> MHHHHHHHHTFTRYSRLRVIAEIRHGDIFHSANIVSSIEFDRDDELFATAGVSRCIKVFDFSSVVNEPADMQCPIVEMSTRSKLSCLSWNKHEKNH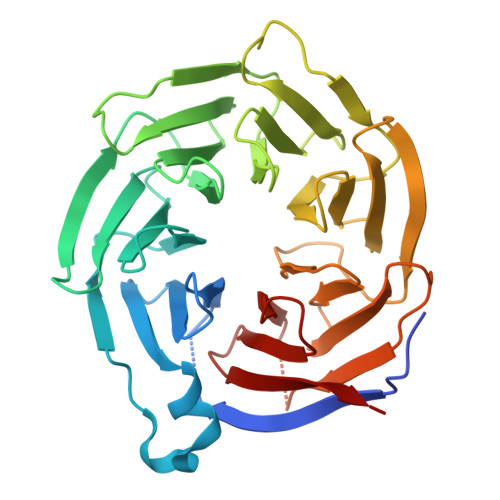IASSDYEGIVTVWDVTTRQSLMEYEEHEKRAWSVDFSRTEPSMLVSGSDDCKVKVWCTRQEASVINIDMKANICCVKYNPGSSNYIAVGSADHHIHYYDLRNISQPLHVFSGHKKAVSYVKFLSNNELASASTDSTLRLWDVKDNLPVRTFRGHTNEKNFVGLTVNSEYLACGSETNEVYVYHKEITRPVTSHRFGSPDMDDAEEEAGSYFISAVCWKSDSPTMLTANSQGTIKVLVLAA> MRGSHHHHHHGL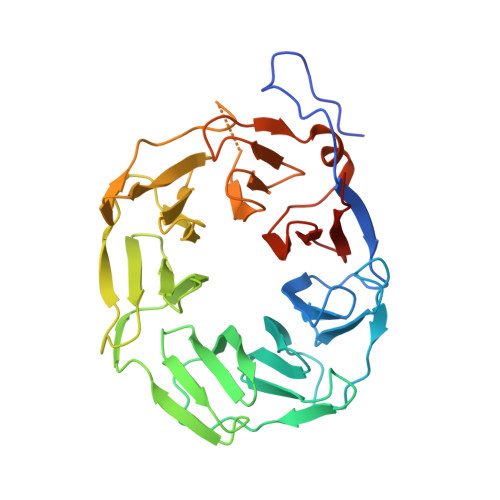VPRGSIPALDYNPWEAIQLPTTATILDMSFIDRHHGWLVGVNATLMETRDGGQTWEPRTLVLDHSDYRFNSVSFQGNEGWIVGEPPIMLHTTDGGQSWSQIPLDPKLPGSPRLIKALGNGSAEMITNVGAIYRTKDSGKNWQALVQEAIGVMRNLNRSPSGEYVAVSSRGSFYSTWEPGQTAWEPHNRTTSRRLHNMGFTPDGRLWMIVNGGKIAFSDPDNSENWGELLSPLRRNSVGFLDLAYRTPNEVWLAGGAGALLCSQDGGQTWQQDVDVKKVPSNFYKILFFSPDQGFILGQKGILLRYVTDLTAAPA[(1R,2R,3R,4R,5S)-2-(hydroxymethyl)-3,4,5-tris(oxidanyl)cyclohexyl]sulfamic 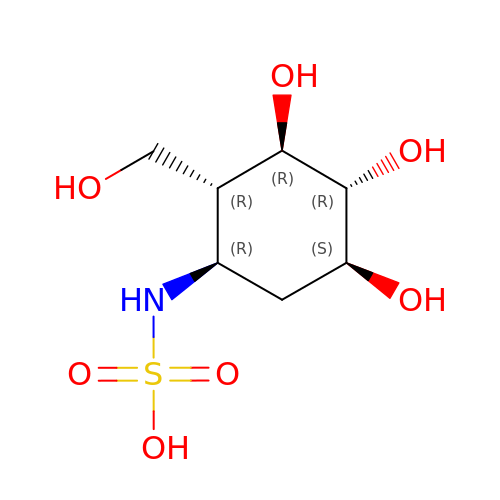acid | C7 H15 N O7 S | QOECHHYORUOADE-PJEQPVAWSA-N>MRIIMPVEFSRIVRDVERLIAVEKYSLQGVVDGDKLLVVGFSEGSVNAYLYDGGETVKLNREPINSVLDPHYGVGRVILVRDVSKGAEQHALFKVNTSRPGEEQRLEAVKPMRILSGVDTGEAVVFTGATEDRVALYALDGGGLRELARLPGFGFVSDIRGDLIAGLGFFGGGRVSLFTSNLSSGGLRVFDSGEGSFSSASISPGMKVTAGLETAREARLVTVDPRDGSVEDLELPSKDFSSYRPTAITWLGYLPDGRLAVVARREGRSAVFIDGERVEAPQGNHGRVVLWRGKLVTSHTSLSTPPRIVSLPSGEPLLEGGLPEDLRRSIAGSRLVWVESFDGSRVPTYVLESGRAPTPGPTVVLVHGGPFAEDSDSWDTFAASLAAAGFHVVMPNYRGSTGYGEEWRLKIIGDPCGGELEDVSAAARWARESGLASELYIMGYSYGGYMTLCALTMKPGLFKAGVAGASVVDWEEMYELSDAAFRNFIEQLTGGSREIMRSRSPINHVDRIKEP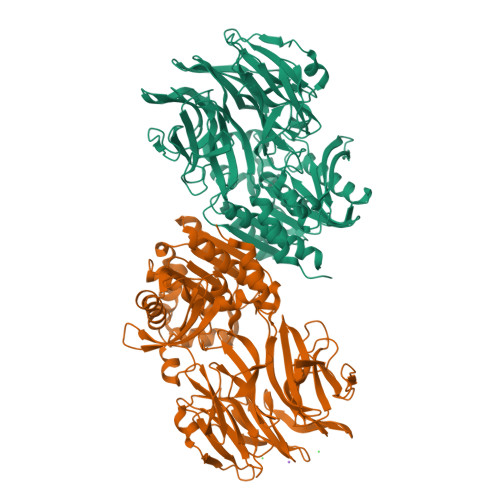LALIHPQNNSRTPLKPLLRLMGELLARGKTFEAHIIPDAGHAINTMEDAVKILLPAVFFLATQRERR[4x]> MEWSWVFLFFLSVTTGVHSWELTILHTNDVHSRLEQTSEDSSKCVDASRCMGGVARLFTKVQQIRRAEPNVLLLDAGDQYQGTIWFTVYKGAEVAHFMNALRYDAMAL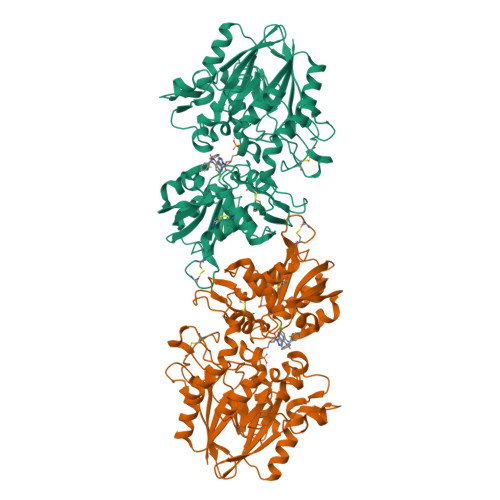GNHEFDNGVEGLIEPLLKEAKFPILSANIKAKGPLASQISGLYLPYKVLPVGDEVVGIVGYTSKETPFLSNPGTNLVFEDEITALQPEVDKLKTLNVNKIIALGHSGFEMDKLIAQKVRGVDVVVGGHSNTFLYTGNPPSKEVPAGKYPFIVTSDDGRKVPVVQAYAFGKYLGYLKIEFDERGNVISSHGNPILLDSSIPEDPSIKADINKWRIKLDDYSTQELGKTIVYLDGSSQSCRFRECNMGNLICDAMINNNLRHTDEMFWNHVSMCILNGGGIRSPIDERNDGTITWENLAAVLPFGGTFDLVQLKGSTLKKAFEHSVHRYGQSTGEFLQVGGIHVVYDLSRKPGDRVVKLDVLCTKCRVPSYDPLKMDEVYKVILPNFLANGGDGFQMIKDELLRHDSGDQDINVVSTYISKMKVIYPAVEGRIKFSGGGGAGGGGHHHHHH>[2x]MQTGFNLSIDTVEGNPGS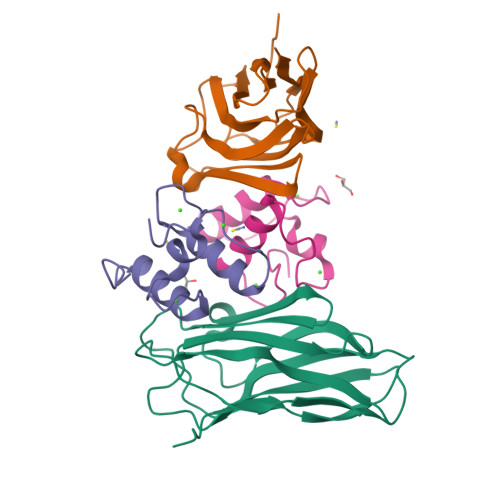SVVVPVKLSGISKNGISTADFTVTYDATKLEYISGDAGSIVTNPGVNFGINKESDGKLKVLFLDYTMSTGYISTDGVFANLNFNIKSSAAIGSKAEVSISGTPTFGDSTLTPVVAKVTNGAVNLE;>KPGDVDGNGSININDFALMRNYLLGNLKDFPAEDDIKAGDLNGDKSINSLDFAIMRMYLLGMITKFSV[2x]>MTADELVFFVNGKKVVEKNADPETTLLAYLRRKLGLRGTKLGCGEGGCGACTVMLSKYDRLQDKIIHFSANACLAPICTLHHVAVTTVEGIGSTKTRLHPVQERIAKSHGSQCGFCTPGIVMSMYTLLRNQPEPTVEEIEDAFQGNLCRCTGYRPILQGFRTFAKNGGCCGGNGNNPNCCMNQKKDHTVTLSPSLFNPEEFMPLDPTQEPIFPPELLRLKDVPPKQLRFEGERVTWIQASTLKELLDLKAQHPEAKLVVGNTEIGIEMKFKNQLFPMIICPAWIPELNAVEHGPEGISFGAACALSSVEKTLLEAVAKLPTQKTEVFRGVLEQLRWFAGKQVKSVASLGGNIITASPISDLNPVFMASGTKLTIVSRGTRRTVPMDHTFFPSYRKTLLGPEEILLSIEIPYSREDEFFSAFKQASRREDDIAKVTCGMRVLFQPGSMQVKELALCYGGMADRTISALKTTQKQLSKFWNEKLLQDVCAGLAEELSLSPDAPGGMIEFRRTLTLSFFFKFYLTVLKKLGKDSKDKCGKLDPTYTSATLLFQKHPPANIQLFQEVPNGQSKEDTVGRPLPHLAAAMQASGEAVYCDDIPRYENELFLRLVTSTRAHAKIKSIDVSEAQKVPGFVCFLSADDIPGSNETGLFNDETVFAKDTVTCVGHIIGAVVADTPEHAERAAHVVKVTYEDLPAIITIEDAIKNNSFYGSELKIEKGDLKKGFSEADNVVSGELYIGGQDHFYLETHCTIAIPKGEEGEMELFVSTQNAMKTQSFVAKMLGVPVNRILVRVKRMGGGFGGKETRSTLVSVAVALAAYKTGHPVRCMLDRNEDMLITGGRHPFLARYKVGFMKTGTIVALEVDHYSNAGNSRDLSHSIMERALFHMDNCYKIPNIRGTGRLCKTNLSSNTAFRGFGGPQALFIAENWMSEVAVTCGLPAEEVRWKNMYKEGDLTHFNQRLEGFSVPRCWDECLKSSQYYARKSEVDKFNKENCWKKRGLCIIPTKFGISFTVPFLNQAGALIHVYTDGSVLVSHGGTEMGQGLHTKMVQVASKALKIPISKIYISETSTNTVPNSSPTAASVSTDIYGQAVYEACQTILKRLEPFKKKNPDGSWEDWVMAAYQDRVSLSTTGFYRTPNLGYSFETNSGNAFHYFTYGVACSEVEIDCLTGDHKNLRTDIVMDVGSSLNPAIDIGQVEGAFVQGLGLFTLEELHYSPEGSLHTRGPSTYKIPAFGSIPTEFRVSLLRDCPNKKAIYASKAVGEPPLFLGASVFFAIKDAIRAARAQHTNNNTKELFRLDSPAT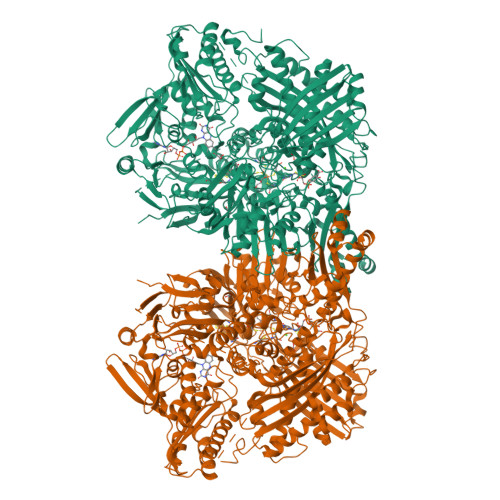PEKIRNACVDKFTTLCVTGAPGNCKPWSLRV[2x]>[4x]MKFRRSGRLVDLTNYLLTHPHELIPLTFFSERYESAKSSISEDLTIIKQTFEQQGIGTLLTVPGAAGGVKYIPKMKQAEAEEFVQTLGQSLANPERILPGGYVYLTDILGKPSVLSKVGKLFASVFAEREIDVVMTVATKGIPLAYAAASYLNVPVVIVRKDNKVTEGSTVSINYVSGSSNRIQTMSLAKRSMKTGSNVLIIDDFMKAGGTINGMINLLDEFNANVAGIGV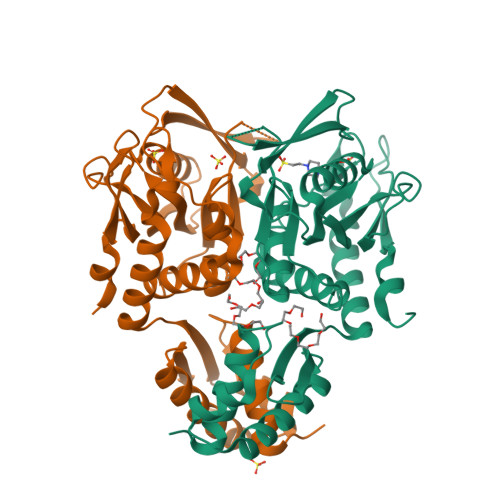LVEAEGVDERLVDEYMSLLTLSTINMKEKSIEIQNGNFLRFFKDNLLKNGETESHHHHHH> GAMAMNDLTLHYLYDPLCGWCYGASPLLAAACEVTGLDVRLHGGGMMTDANRQPVGAGLRHYVMPHDLRIAQLTGQPFGKDYFDGLLRDTSAVFDSAPPTAAVLAAEALDGLGAAMLARIQRAHYVEGRRIAERPVLLELGAELGLGEGFAEAFDACSGEPLRAHFADSRRLMNRLGAAGFPTFALERDGRLQV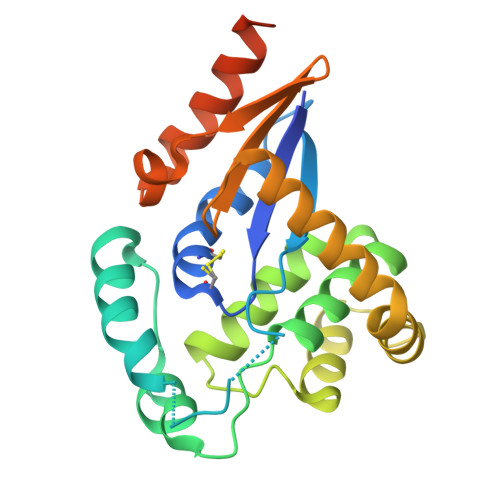LDTGRYLGQPDDWRAFLETQLRLAGGSGAVGGAAAPLCRIDGCA1-[3-methyl-4-({3-[2-(methylamino)pyrimidin-4-yl]pyridin-2-yl}oxy)phenyl]-3-[3-(trifluoromethyl)phenyl]urea 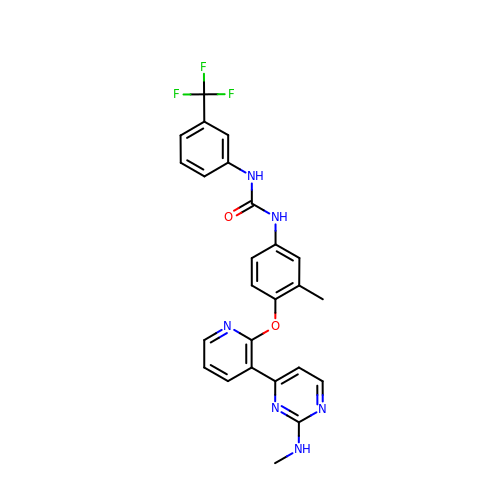| C25 H21 F3 N6 O2 | INFGJUQNPPGDNS-UHFFFAOYSA-N> AERPTLPIPDLLTTDARNRIQLTIGAGQSTFGGKTATTWGYNGNLLGPAVKLQRGKAVTVDIYNQLTEETTLHWHGLEVPGEVDGGPQGIIPPGGKRSVTLNVDQPAATCWFHPHQHGKTGRQVAMGLAGLVVIEDDEILKLMLPKQWGIDDVPVIVQDKKFSADGQIDYQLDVMTAAVGWFGDTLLTNGAIYPQHAAPRGWLRLRLLNGCNARSLNFATSDNRPLYVIASDGGLLPEPVKVSELPVLMGERFEVLVEVNDNKPFDLVTLPVSQMGMAIAPFDKPHPVMRIQPIAISASGALPDTLSSLPALPSLEGLTVRKLQLSMDPMLDMMGMQMLMEKYGDQAMAGMDHSQMMG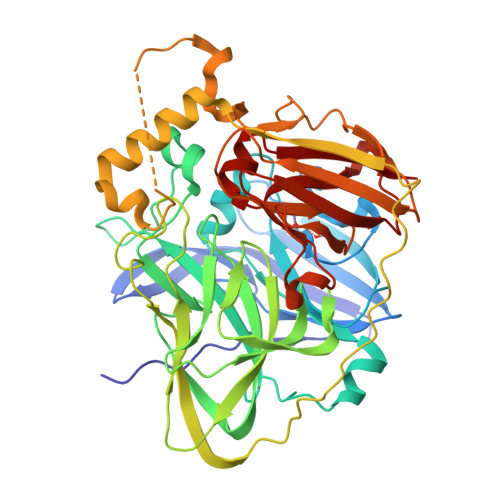HMGHGNMNHMNHGGKFDFHHANKINGQAFDMNKPMFAAAKGQYERWVISGVGDMMLHPFHIHGTQFRILSENGKPPAAHRAGWKDTVKVEGNVSEVLVKFNHDAPKEHAYMAHSHLLEHQDTGMMLGFTVG> GSHVMDSSSMSVENANEVMKYYDTSLKILKDLVNENEIKAVLGYLDQKMPVDSLPVVSQPVVSV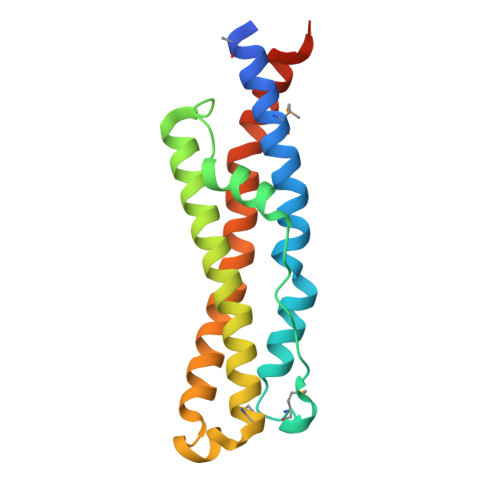QDTVFVSNPGNYFSENDRQNLKENYGRLFRSISAFYENYKTYRLYMQDQSYKKDNNALADKIRKEELLLSIALSEYKQVIFDILTPIVEGAKITLTPIKGNVKDK Toward this goal, the present work describes the use of bovine pancreatic ribonuclease (RNase A) crystals with a pore size of 4 nm (P3221 space group) for fixing [Rh2(OAc)4] and developing a heterogeneous catalyst to perform reactions in an aqueous medium. The structure of the [Rh2(OAc)4]/RNase A adduct was investigated by X-ray crystallography: the metal complex structure remains unperturbed upon protein binding. Structural analysis demonstrates that 1 h of soaking is sufficient to metalate the protein and that the crystal packing does not influence the binding of the metal compound to RNase A: two binding sites were identified for the metal compound, close to the His105 and His119 side chains, in agreement with that observed using RNase A crystals in a different crystal form. Overall, our findings demonstrate that the dirhodium paddlewheel complexes can be fixed in porous biomolecule crystals, like those of RNase A, to prepare biohybrid materials for catalytic applications.

Crystals of the adduct with [Rh2(OAc)4] were formed via soaking using RNase A crystals grown at pH 5.2. To characterize the metal binding process within the protein crystals, X-ray diffraction data were collected on RNase A crystals exposed to [Rh2(OAc)4] for different soaking times (1, 2, and 6 h). Hence, three different structures of the [Rh2(OAc)4]/RNase A adduct in the P3221 space group were solved. In all of the structures, two binding sites for the metal compound were observed, close to His105 and His119 side chains, as observed in previous reports. Close to the His105 side chain, [Rh2(OAc)4] (occupancy = 0.70–0.78) is linked to the Nε atom of the imidazole ring and to a Cl– ion through its axial positions. The axial binding of the Cl– ion to the dirhodium core is not surprising considering the high concentration of NaCl in the crystallization conditions. A Cl– ion is found at the axial position of the dirhodium center also in the case of the metal-containing fragment bound to the His119 side chain. However, at this site, the remaining axial position of the dirhodium core (occupancy = 0.50–0.55) is coordinated to the Nδ atom of the His imidazole ring, and the dimetallic compound is equatorially coordinated by three acetate ligands and two water molecules. In the structure collected after 1 h of soaking, a double conformation of the His119 side chain is observed. In conclusion, considering that the occupancy of dirhodium does not significantly change between 1 and 6 h of soaking, it can be assumed that 1 h of soaking is sufficient to metalate the protein in the solid state.

> KETAAAKFERQHMDSSTSAASSSNYCNQMMKSRNLTKDRCKPVNTFVHESLADVQAVCSQKNVACKNGQTNCYQSYSTMSITDCRETGSSKYPNCAYKTTQANKHIIVACEGNPYVPVHFDASV>[4x]GDDCEDLHLGNLAHYPNVLKGTFPTESQVLELGETLEITPELLNPEGATYSWLVNGKEYSTEPTFSYKIDNPCRADLSCIIKNKYGKVEMSTSFSSNHNFSKGFFYVADGTFNFYDTEKKTAYQDCYASLNAGKTLGIGNYDSANIIHSNGKFYLLVGTSTSNRDHFYIVDAKTLYYENSAVVGANLSGLTILNEQYGLVTGDGIRRIDLKSLNNVRIKNERLLCFYNSIIYNGKVLSNDTYKDE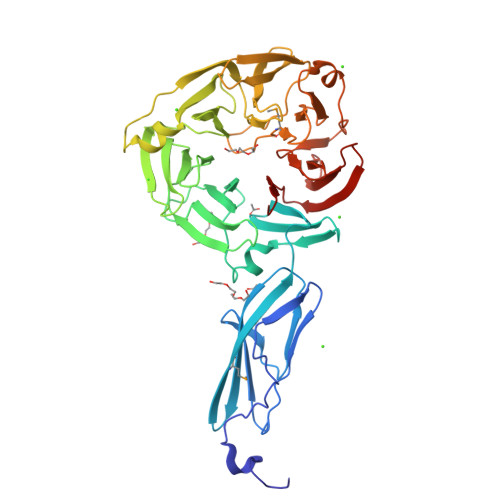SKVKYYDVNELIAAKEGEAPAVTELDIIQKQKINFVLAKDGNVYTLESADNGCNIVKIKNDFTLEKVFANFQPAKGPYHSSPTIGMVASETENIIYLVSTDGAIYKYILGDSDSLKAPFIAAESGVSITAPLQLNQQSGELYVTYTEERKDESKIVVYSKDGKVLHTVDCGESVPSQILFNN> SPSAEACGYSDRVAQLTIGNSTITTQEAANIIVGYGEWPSYCSDSDATAVDKPTRPDVSVNRFYTLDTKLWEKSSKGW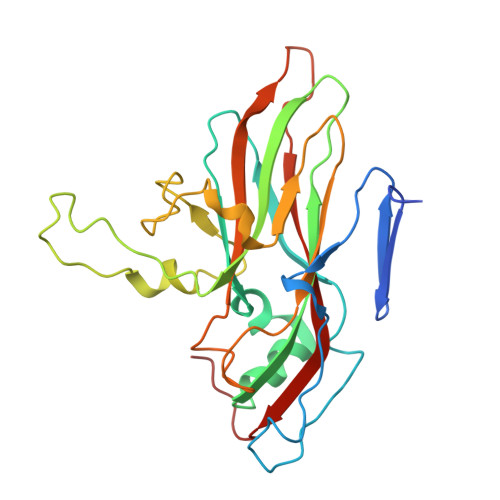YWKFPDVLTETGVFGQNAQFHYLYRSGFCIHVQCNASKFHQGALLVAVLPEYVIGTVAGGTGTEDTHPPYKQTQPGADGFELQHPYVLDAGIPISQLTVCPHQWINLRTNNCATIIVPYINALPFDSALNHCNFGLLVVPISPLDYDQGATPVIPITITLAPMCSEFAGLRQAVTQ> AQTINLQLEGMDCTSCASSIERAIAKVPGVQSCQVNFALEQAVVSYHGETTPQILTDAVER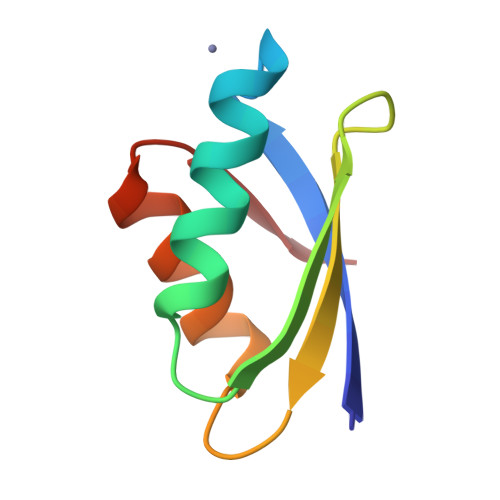AGYHARVL The NS1 protein of influenza virus is an important virulence factor and has been demonstrated to interact with a wide variety of viral and cellular biomolecules. The effector domain (ED) of the influenza virus virulence factor NS1 is capable of interaction with a variety of cellular and viral targets, although regulation of these events is poorly understood. Furthermore, both domains form homodimers in vitro. While the conformation of the RBD dimer appears to be conserved, two forms of the ED dimer have been proposed: the strand–strand dimer and the helix–helix dimer.

In this paper, we report a third X-ray crystallographic structure of the PR8 NS1 ED containing the W187A mutation. A new condition for crystallization of this protein [0.1 M Bis-Tris pH 6.0, 0.2 M NaCl, 22%(w/v) PEG 3350, 20 mM xylitol] was discovered using the hanging-drop vapour-diffusion method. Diffraction data extending to 1.8 Å resolution were collected from a crystal grown in the presence of 40 mM thieno[2,3-­b]pyridin-2-ylmethanol. The novel crystal form of PR8 NS1 ED (W187A) shows the α/β fold common to all structures of NS1 ED. The introduction of a W187A mutation into the ED induces a monomeric phenotype and, intriguingly, two crystal structures of the PR8 NS1 ED containing this mutation also exhibit this strand–strand interface. However, it is intriguing to observe that the strand–strand dimer is conserved among all three PR8 NS1 ED (W187A) structures that have now been solved. Therefore, since the PR8 NS1 ED W187A mutant is monomeric in vitro, it appears highly likely that the helix–helix dimer is the predominant interface for ED homodimerization. The partial con­servation of the strand–strand packing interface indicates that while it may not allow ED dimerization, extension of the β-sheet is a possible method of interaction with cellular and viral binding partners.

> MTMASVPASRYLTDMTLEEMSRDWSMLIPKQKVAGPLCIRMDQAIMDKNIILKANFSVIFDRLETLILLRAFTEEGAIVGEISPLPSLPGHTAEDVKNAVGVLIGGLEANDNTVRVSETLQRFAWRSSNENGRPPLTPKQKREMAGTIRSEV>GMSWEKSGKEGSLLRWYDVMEAERYEYTVGPAGEQFFNGLKQNKIIGSKCSKCGRIFVPARSYCEHCFVKIENYVEINKDEAYVDSYTIIYND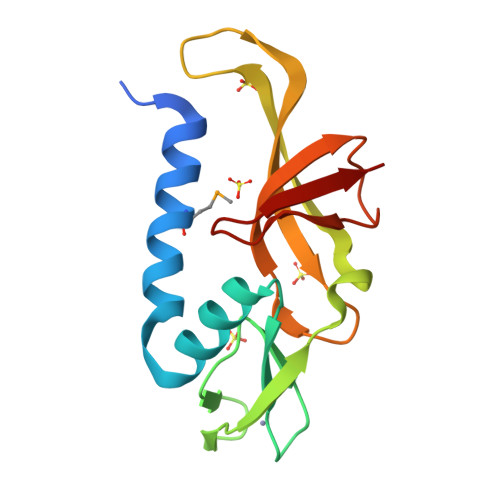DEGNKLAQPVYIALIRFPNIEGGLLCYAEGNVKVGAKAKILSFQWPLRVKVD[2x]>[2x]MHHHHHHMLENKLGIINQLELNRVEERVSKENAKRLYDSGDIDRIEVGTFKGLSYIHNYLFEDIYEFAGKVRSQNISKGNFRFAPVMYLEIALEHIDKMPQRNLDEIVAKYVEMNIAHPFREGNGRATRIWLDLILKKELKRVVDWNLINKEDYLSAMERSPVKDLEIKYLISNALTDKINDREIFMKGIDISYYYEGYTEYNVDEL

The most frequent PTM reaction catalyzed by FIC enzymes is the addition of AMP using ATP as a cofactor, coined AMPylation or adenylylation. Enterococcus faecalis FIC belongs to class III FIC proteins, which are comprised of a single FIC domain and carry an autoinhibitory glutamate in their C-terminal α-helix. We discover that EfFIC has both AMPylation and deAMPylation activities borne by the same active site. Furthermore, the conserved glutamate implements a Ca2+-controlled metal switch that tunes the balance between these activities without conformational change.

To gain further insight into the enzymatic properties of EfFIC, we solved the crystal structure of EfFICWT bound to AMP, used as a surrogate of the product of the AMPylation reaction. Electron-rich density was observed next to AMP in the active site, ascribed to a calcium ion present in the crystallization solution to the exclusion of all other metal ions. Ca2+ binds to six oxygen atoms, including a phosphate oxygen of AMP, the carboxylate oxygen of the acidic residue in the FIC motif (Glu115), and three water molecules, one of which is also bound to the inhibitory glutamate (Glu190), with the seventh ligand missing. The position of Ca2+ in the EfFICWT-AMP structure is shifted with respect to that of Mg2+ observed in other FIC protein structures in complex with ATP, raising the intriguing possibility that it may support an alternative biochemical activity. The nucleophilic water molecule is readily identified as the missing ligand needed to complete the heptahedral coordination sphere of Ca2+ in the EfFIC-AMP-Ca2+ structure, where it would be precisely positioned for in-line nucleophilic attack. Based on the observations that the α- and β-phosphates of ATP bind with canonical positions to wild-type EfFIC and that AMPylation is potentiated by mutation of the conserved glutamate in various FIC proteins, we propose that the primary role of this glutamate in AMPylation is to mitigate the efficiency of this reaction in the presence of Mg2+, rather than to fully repress it, possibly in order to match AMPylation and deAMPylation efficiencies. In the deAMPylation mechanism depicted in Fig. 5 (see also discussion in Supplementary Discussion and Supplementary Fig. 3), the conserved glutamate activates a water molecule for nucleophilic attack of the phosphorus of the AMP moiety of the AMPylated substrate, and the invariant histidine generates the free hydroxyl group in the protein residue by giving up a proton, as also proposed in ref.> MKCLVTGGN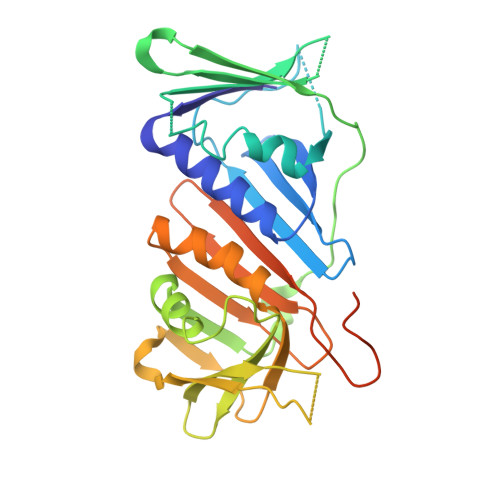VKVLGKAVHSLSRIGDELYLEPLEDGLSLRTVNSSRSAYACFLFAPLFFQQYQAATPGQDLLRCKILMKSFLSVFRSLAMLEKTVEKCCISLNGRSSRLVVQLHCKFGVRKTHNLSFQDCESLQAVFDPASCPHMLRAPARVLGEAVLPFSPALAEVTLGIGRGRRVILRSYHEEEADSTAKAMVTEMCLGEEDFQQLQAQEGVAITFCLKEFRGLLSFAESANLNLSIHFDAPGRPAIFTIKDSLLDGHFVLATLSDTDSGTTSTSLEVLFQGPLSGSGGHHHHHH>[8x]GSSLISA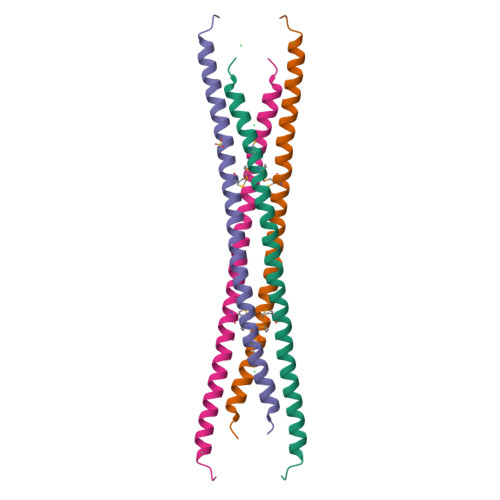VSDKLRWRMKEEMDRAQAELNALKRTEEDLKKGHQKLEEMVTRLDQEVAEVDKNIELLKKKDEELSSALEK3-PHOSPHONOPROPANOIC 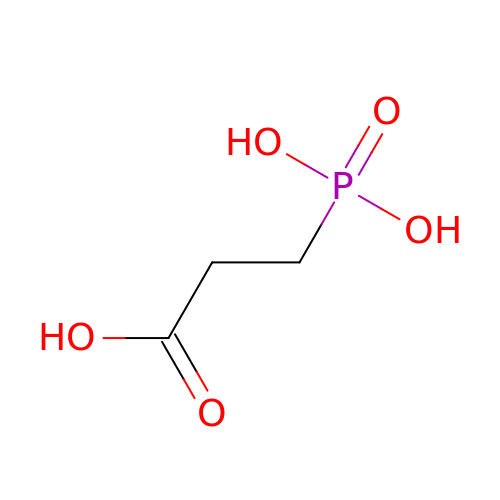ACID | C3 H7 O5 P | NLBSQHGCGGFVJW-UHFFFAOYSA-N>[2x]GGHMAKHHPDLIFCRKQAGVAIGRLCEKCDGKCVICDSYVRPSTLVRICDECNYGSY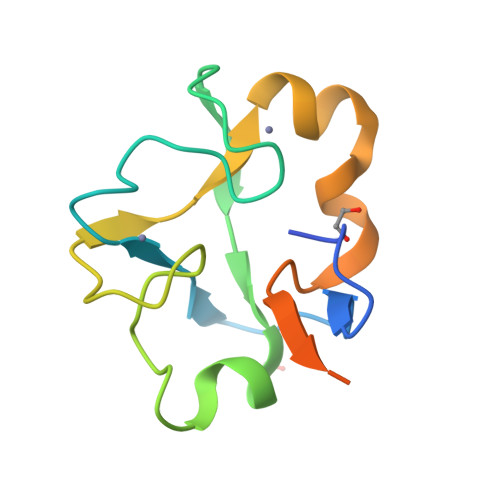QGRCVICGGPGVSDAYYCKECTIQEKDRDGCPKIVNLGSSKTDLFYERKKYGFKKR>[2x]MIKLVTFDLDDTLWDTAPAIVGAEAALRDWLAEQAPKLGPVPVEHLWEIRSRLLDEDPSFKHRISALRRRVLFHALEDAGYDSD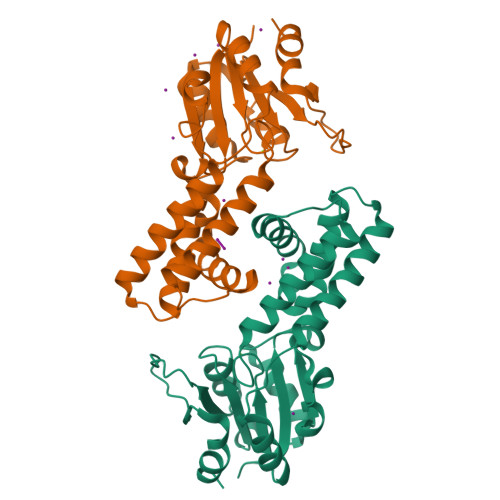EAQQLADESFEVFLHGRHQVQIFPEVQPTLEILAKTFTLGVITNGNADVRRLGLADYFAFALCAEDLGIGKPDPAPFLEALRRAKVDASAAVHVGDHPSDDIAGAQQAGMRAIWYNPQGKAWDADRLPDAEIHNLSQLPEVLARWA1-[(3~{R})-3-(4-azanyl-3-iodanyl-pyrazolo[3,4-d]pyrimidin-1-yl)piperidin-1-yl]propan-1-one 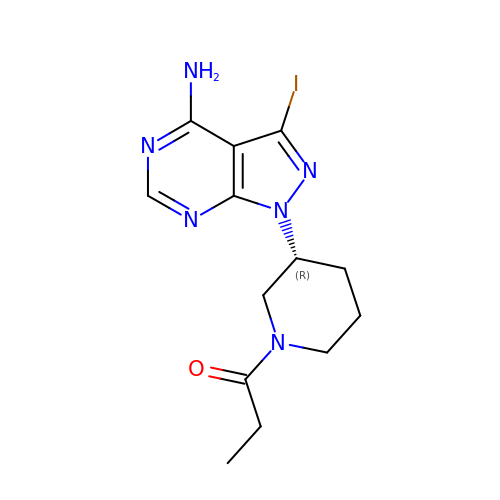| C13 H17 I N6 O | CBMKHVATJGHRQV-MRVPVSSYSA-N>[2x]MANKTYKIGKNAGYDGCGLCLAAISENEAIKVKYLRDICPDYDGDDKAEDWLRWGTDSRVKAAALEMEQYAYTSVGMASCWEFVEL

Anti-CRISPRs (Acrs) are natural inhibitors of bacteria’s CRISPR-Cas systems, and have been developed as a safeguard to reduce the off-target effects of CRISPR gene-editing technology. Structural studies show that AcrIIC1 can directly bind to the conserved HNH nuclease domain of Cas9 to abolish its DNA cleavage activity. Among the different Acr proteins characterized so far, AcrIIC1, a broad-spectrum inhibitor against diverse type II-C Cas9 orthologs, is one of the most promising engineering candidates to target the desired Cas98,14. In this work, we report the discovery of a redox switch for NmeAcrIIC1, which regulates NmeAcrIIC1’s monomer-dimer interconversion and inhibitory activity on Cas9.

Fortunately, we managed to grow protein crystals formed by the oxidized NmeAcrIIC1 and solve the crystal structure of the dimer with a resolution of 1.61 Å by using X-ray crystallography. In the dimeric structure, one of the protomers is rotated roughly 180 degrees relative to the other partner, which then allows for the dimerization via two intermolecular disulfide bonds. Strikingly, the two subunits assemble mainly through two parallel intermolecular disulfide bonds formed by Cys17 and Cys80, but not hydrophobic or electrostatic interaction that is commonly observed in mediating protein–protein interaction. The subunit orientation of the dimer is restricted to a great extent by the two intermolecular disulfide bonds, shown in Fig. 3c, d. Each subunit of the dimeric form aligns with the reduced monomeric form of NmeAcrIIC1 with a small RMSD of 0.68 and 0.73 Å, respectively. Second, by examining the electron density map of the oxidized NmeAcrIIC1, we observed that both of the intermolecular disulfide bonds are not fully occupied, indicative of dynamic short-lived chemical groups. Second, the estimated rotational correlation time (Τc) for the oxidized dimer is almost twice as that for the reduced monomer (11.6 versus 6.0 ns), whereas the trends of 15N backbone relaxation data of R1, R2, and Het-NOE align well between the two states on a residue-by-residue base, which reveals a rigid dimer with restricted orientation for each subunit but lacking large interfacial surface that is supposed to alter the dynamic properties of the residues involved. Together, the CSD and 15N relaxation data for both forms of NmeAcrIIC1 in solution strongly support the crystal structure, stating that the crystal structure of the oxidized dimer can reliably represent the dimer’s behavior in solution. Importantly, compared with the structure of NmeAcrIIC1’s complex with NmeHNH, the counterpart subunit of dimeric NmeAcrIIC1 occupies the position of the NmeHNH, burying the “hot spot” residue Ser79, thereby inhibiting the interaction between NmeAcrIIC1 with NmeHNH through steric hindrance. Thus, the dimeric structure rationalizes how oxidization and dimerization of NmeAcrIIC1 result in the disruption of NmeHNH binding and the loss of inhibitory activity against Cas9.> SNGIEASLLTDPKDVSGRTVDYIIAGGGLTGLTTAARLTENPNISVLVIESGSYESDRGPIIEDLNAYGDIFGSSVDHAYETVELATNNQTALIRSGNGLGGSTLVNGGTWTRPHKAQVDSWETVFGNEGWNWDNVAAYSLQAERARAPNAKQIAAGHYFNASCHGVNGTVHAGPRDTGDDYSPIVKALMSAVEDRGVPTKKDFGCGDPHGVSMFPNTLHEDQVRSDAAREWLLPNYQRPNLQVLTGQYVGKVLLSQNGTTPRAVGVEFGTHKGNTHNVYAKHEVLLAAGSAVSPTILEYSGIGMKSILEPLGIDTVVDLPVGLNLQDQTTATVRSRITSAGAGQGQAAWFATFNETFGDYSEKAHELLNTKLEQWAEEAVARGGFHNTTALLIQYENYRDWIVNHNVAYSELFLDTAGVASFDVWDLLPFTRGYVHILDKDPYLHHFAYDPQYFLNELDLLGQAAATQLARNISNSGAMQTYFAGETIPGDNLAYDADLSAWT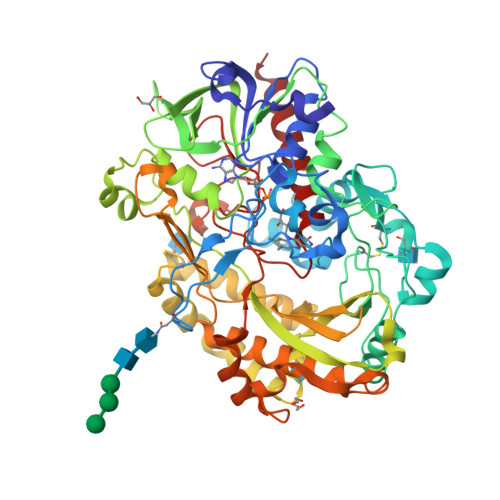EYIPYHFRPNYHGVGTCSMMPKEMGGVVDNAARVYGVQGLRVIDGSIPPTQMSSHVMTVFYAMALKISDAILEDYASMQ>[2x]MAKHLFTSESVSEGHPDKIADQISDAVLDAILEQDPKARVACETYVKTGMVLVGGEITTSAWVDIEEITRNTVREIGYVHSDMGFD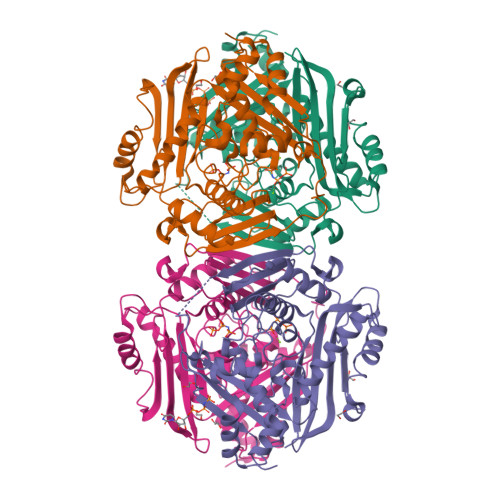ANSCAVLSAIGKQSPDINQGVDRADPLEQGAGDQGLMFGYATNETDVLMPAPITYAHRLVQRQAEVRKNGTLPWLRPDAKSQVTFQYDDGKIVGIDAVVLSTQHSEEIDQKSLQEAVMEEIIKPILPAEWLTSATKFFINPTGRFVIGGPMGDCGLTGRKIIVDTYGGMARHGGGAFSGKDPSKVDRSAAYAARYVAKNIVAAGLADRCEIQVSYAIGVAEPTSIMVETFGTEKVPSEQLTLLVREFFDLRPYGLIQMLDLLHPIYKETAAYGHFGREHFPWEKTDKAQLLRDAAGLK>[2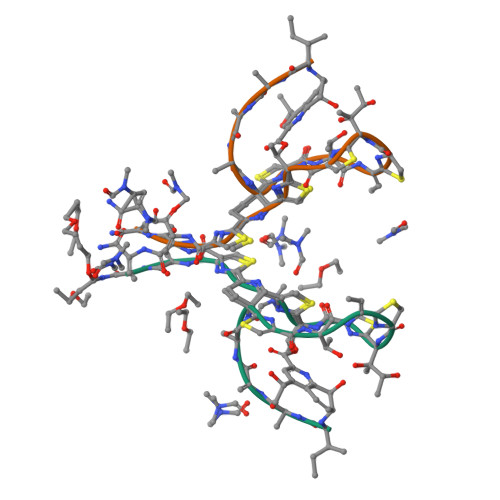x]XIASASCTTCICTCSCSSX N-[(2R)-3-(3-cyanophenyl)-1-oxo-1-(pyrrolidin-1-yl)propan-2-yl]-8-fluoro-1,2,3,4-tetrahydroisoquinoline-6-sulfonamide 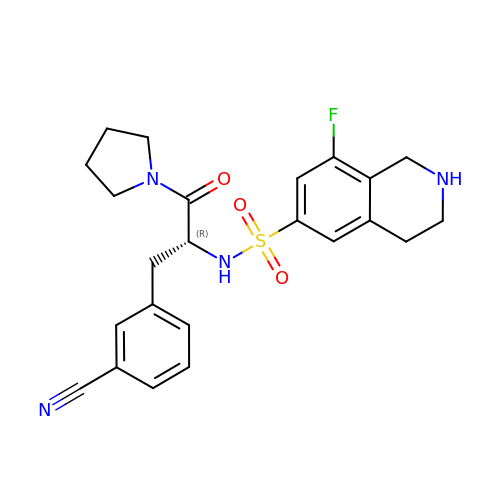| C23 H25 F N4 O3 S | HMBXWXQQVHJMOO-JOCHJYFZSA-N>MKKIVLYGGQFNPIHTAHMIVASEVFHELQPDEFYFLPSFMSPLKKHHDFIDVQHRLTMIQMIIDELGFGDICDDEIKRGGQSYTYDTIKAFKEQHKDSELYFVIGTDQYNQLEKWYQIEYLKEMVTFVVVNR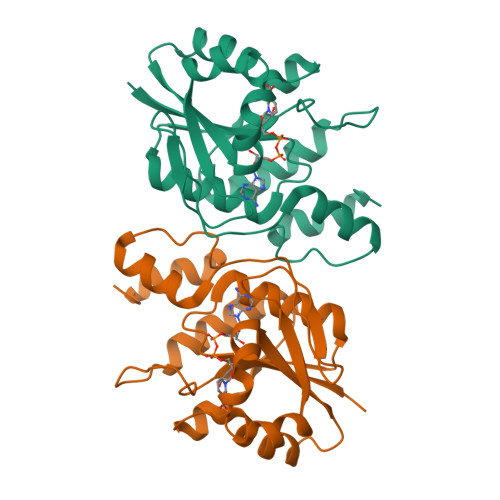DKNSQNVENAMIAIQIPRVDISSTMIRQRVSEGKSIQVLVPKSVENYIKGEGLYEH[2x]> MSIDKSYCGFIAIVGRPNVGKSTLLNKLLGQKISITSRKAQTTRHRIVGIHTEGAYQAIYVDTPGLHMEEKRAINRLMNKAASSSIGDVELV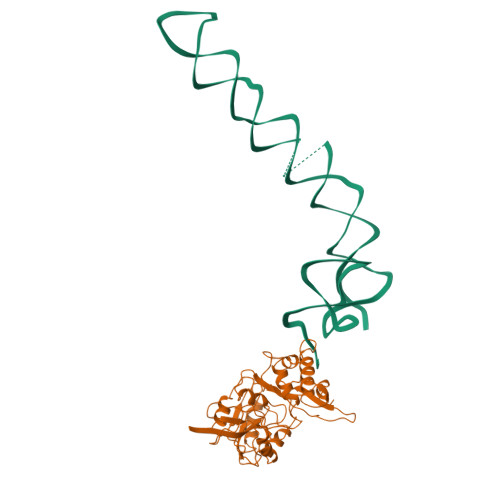IFVVEGTRWTPDDEMVLNKLREGKAPVILAVNKVDNVQEKADLLPHLQFLASQMNFLDIVPISAETGLNVDTIAAIVRKHLPEATHHFPEDYITDRSQRFMASEIIREKLMRFLGAELPYSVTVEIERFVSNERGGYDINGLILVEREGQKKMVIGNKGAKIKTIGIEARKDMQEMFEAPVHLELWVKVKSGWADDERALRSLGYVDDL> MENTLGEGSTVNASVDVDQHGNDNNSDSNANAAVAGVANTDTAGEESQQQDESLKDEATVPNTRDAESEAITVTAKQQPTMQANKLDSQETPSTEESRAQNVFGQDNEDSDNLFGETESSVSNNEANTPSIPTNPVDNENNKPAIKEDSTIQDSNGDVKNMEDVKIQKEEEPENNTVIEGVKEESQPDENTKEMDEVEEDDEDDDQPMISPDNSIFGDTKSESKQLGNTSSVANTPSEIPDAHKAEQEDIIEKTESVDKKVDSGEERNEQEREIMNDHSKSANPKKTTITRVEPETFEIPQAHEIVIPSYSKWFNLEKIHSIEVQSLPEFFTNRIPSKTPEVYMRYRNFMVNSYRLNPNEYFSVTTARRNVSGDAAALFRLHKFLTKWGLINYQVDSKLLPKNIEPPLTSQYSTRHDAPRGLFPFESYKPSVQLPDMAKLKKMMNTSDSESTLYKYLKESKRKYDEITHPPSTTDDENGDKNDNGGKMNNEVSTSTSMTGDANLLEEGETSRPLKKVKILEQIDENWSKEDLQKLLKGIQEFGADWYKVAKNVGNKSPEQCILRFLQLPIEDKFLYGDGNGKGDNDNGLGPLKYAPHLPF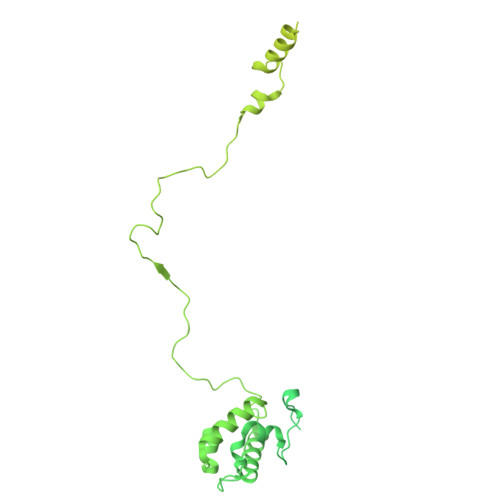SKSENPVLSTIAFLVGLVNPKTVQSMTQRAIQSAESIKSQKEEISDQKPIEHIKEGSEIAISSLGYRSHIFATNEERQMNFLTNELIRLQMEKLDAKLNHLKKLEKFMELERKTLERQQENLLIQRLNFNQNSSKIVNVLSKCLNLISDSNINNSSVAEKEEIRSQIDHFKSMLSKPETLSIGKNPFNKPNIETGENHNGQSISNENDVKPISIEAPQFYRYWSA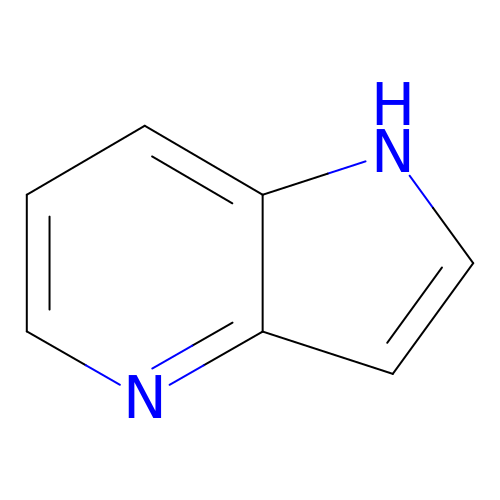1H-pyrrolo[3,2-b]pyridine | C7 H6 N2 | XWIYUCRMWCHYJR-UHFFFAOYSA-N5-(3-(2,6-DICHLORO-4-(4,5-DIHYDRO-2-OXAZOLYL)PHENOXY)PROPYL)-3-METHYL ISOXAZOLE | 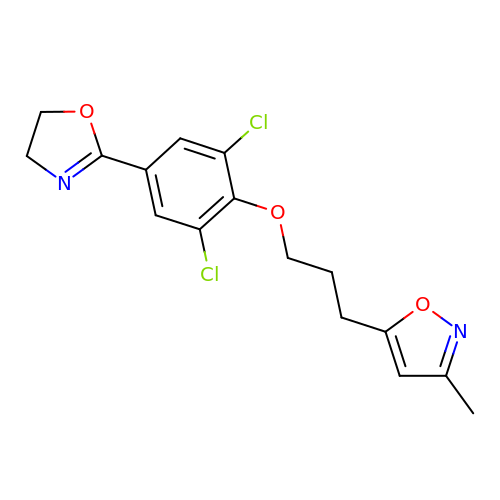C16 H16 Cl2 N2 O3 | TUGBWRGTMLOFAX-UHFFFAOYSA-N5-[1-methyl-5-(1-phenylcyclopropyl)-1,2,4-triazol-3-yl]-3-(1~{H}-pyrazol-4-yl)pyrazin-2-amine | C19 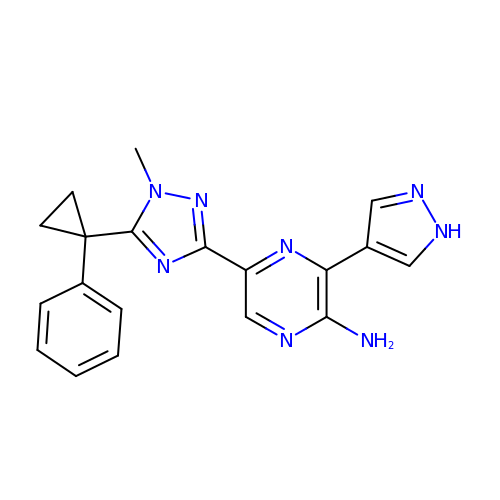H18 N8 | RJOTUMAUCUPABW-UHFFFAOYSA-N> MKLLWQVTVHHHTWNAILLPFVYLTAQVWILCAAIAAAASAGPQNCPSVCSCSNQFSKVVCTRRGLSEVPQGIPSNTRYLNLMENNIQMIQADTFRHLHHLEVLQLGRNSIRQIEVGAFNGLASLNTLELFDNWLTVIPSGAFEYLSKLRELWLRNNPIESIPSYAFNRVPSLMRLDLGELKKLEYISEGAFEGLFNLKYLNLGMCNIKDMPNLTPLVGLEELEMSGNHFPEIRPGSFHGL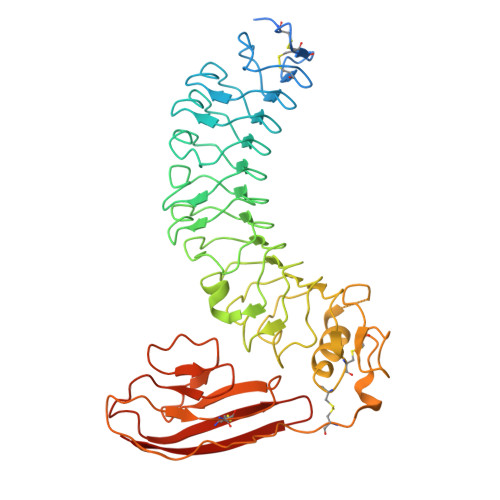SSLKKLWVMNSQVSLIERNAFDGLASLVELNLAHNNLSSLPHDLFTPLRYLVELHLHHNPWNCDCDILWLAWWLREYIPTNSTCCGRCHAPMHMRGRYLVEVDQASFQCSAPFIMDAPRDLNISEGRMAELKCRTPPMSSVKWLLPNGTVLSHASRHPRISVLNDGTLNFSHVLLSDTGVYTCMVTNVAGNSNASAYLNVSTAGTHHHHHH> DEETFEEFTARYEKEFDEAYDLFEVQRVLNNCFSYDLVPAPAVIEKALRAAR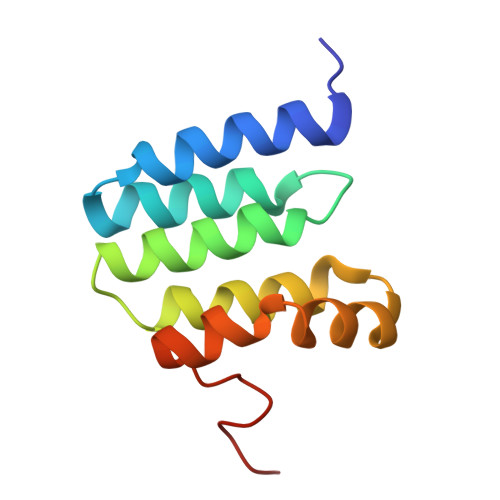RVNDLPTAIRVFEALKYKVENEDQYKAYLDELKDVRQELGVPLKEELFPSSS> GSGHWGAWMPSTISAFEGTCVSIPCRFDFPDELRPAVVHGVWYFNSPYPKNYPPVVFKSRTQVVHESFQGRSRLLGDLGLRNCTLLLSTLSPELGGKYYFRGDLGGYNQYTFSEHSVLDIVNTPNIVVPPEVVAGTEVEVSCMVPDNCPELRPELSWLGHEGLGEPTVLGRLREDEGTWVQVSLLHFVPTREANGHRLGCQAAFPNTTLQFEGYASLDVKYPPVIVEMNSSVEAIEGSHVSLLCGADSNPPPLLTWMRDGMVLREAVAKSLYLDLEEVTPGEDGVYACLAENAYGQDNRTVELSVMYAPWKPTVNGTVVAVEGETVSILCSTQSNPDPILTIFKEKQILATVIYESQLQLELPAVTPEDDGEYWCVAENQYGQRATAFNLSVEFAPIILLESHCAAARDTVQCLCVVKSNPEPSVAFELPSRNVTVNETEREFVYSERSGLLLTSILTIRGQAQAPPRVICTSRNLYGTQSLELPFQGAHRAAAHHHHHH

MAG is a type 1 single-pass transmembrane protein expressed on myelinating oligodendrocytes in the CNS and Schwann cells in the PNS23. Myelin-associated glycoprotein (MAG) adhesion and signalling at the myelin–axon interface regulates the formation and maintenance of myelinated axons, thus playing an important role in the development and function of the nervous system. MAG adhesion maintains the myelin–axon spacing (periaxonal diameter) by interacting with specific neuronal gangliosides (glycolipids), such as the major brain gangliosides GT1b and GD1a. On the basis of the primary sequence its extracellular region is predicted to consist of five Ig domains; an N-terminal V-type Ig domain that is typical for Siglecs and four C2-type Ig domains.

We determined crystal structures of the full extracellular segment of mouse MAG (MAG1–5) in two different crystal forms that diffracted to a maximum resolution of 3.8 and 4.3 Å. These crystals were obtained by enzymatic deglycosylation of MAG1–5 or reductive lysine methylation of glycosylated MAG1–5 (see ‘Methods' section). The structures were solved by molecular replacement with individual Ig domains from homologous proteins. The exceptionally high-solvent content of the two MAG1–5 crystal forms (91 and 85%) aided in obtaining phases of sufficient quality for initial model building (see also Table 1 and ‘Methods' section for details). We observed unmodelled electron density in the 2Fo−Fc and Fo−Fc maps of the deglycosylated MAG1–5 structure close to R118 in the putative ligand-binding site20. Native mass spectrometry of purified MAG1–5 revealed a mixture of free and two ligand-bound MAG1–5 forms with mass differences of 835±2 and 854±2 Da compared with free MAG1–5. The 835 Da ligand possibly corresponds to a tetrasaccharide comprising the aforementioned Neu5Ac-α2,3-Gal-β1,3-GalNAc trisaccharide plus another hexose. The 854 Da ligand might correspond to a similar tetrasaccharide where Neu5Ac is replaced by Neu5Gc, a mammalian sialic acid variant not produced by humans. These ligands are likely co-purified in complex with MAG from the expression medium that contains beef digest (Primatone). The resolution of the MAG1–5–ligand complex (to 3.8 Å) is not sufficient to determine the detailed structure of the bound oligosaccharide. However, the unmodelled electron density is compatible with either of the suggested compounds.>[2x]GASKLRAVLEKLKLSRDDISTAAGMVKGVVDHLLLRLKCDSAFRGVGLLNTGSYYEHVKISAPNEFDVMFKLEVPRIQLEEYSNTRAYYFVKFKRNPKENPLSQFLEGEILSASKMLSKFRKIIKEEINDIKDTDVIMKRKRGGSPAVTLLISEKISVDITLALESKSSWPASTQEGLRIQNWLSAKVRKQLRLKPFYLVPKHAKEGNGFQEETWRLSFSHIEKEILNNHGKSKTCCENKEEKCCRKDCLKLMKYLLEQLKERFKDKKHLDKFSSYHVKTAFFHVCTQNPQDSQWDRKDLGLCFDNCVTYFLQCLRTEKLENYFIPEFNLFSSNLIDKRSKEFLTKQIEYERNNEFPVFDEF

Cyclic GMP-AMP synthase (cGAS) is the most recently identified member of the family of cytosolic DNA sensors. Cytosolic cGAS binds dsDNA and in the presence of ATP and GTP catalyzes the production of the recently characterized second messenger 2′, 3′- cyclic AMP-GMP (cGAMP) which then binds to Stimulator of Interferon Genes (STING). In humans, the binding of the cGAS product to STING causes a conformational change resulting in recruitment of TBK1, and interferon-inducible gene activation and interferon production via IRF3 phosphorylation and nuclear translocation. Activation of cGAS is important in host defense against pathogens, but uncontrolled activation of the cGAS pathway has been implicated in autoinflammatory disease.

Although DNA-binding compounds may indirectly inhibit cGAS activity, to our knowledge no inhibitor shown to bind directly to the cGAS active site has been reported. To discover cGAS active site inhibitors we used NMR screening of a fragment library and identified a compound that binds competitively with cGAMP.>[2x]DPKFQRVALSDGHFIPVLGFGTYAPEEVPKSKAMEATKIAIDAGFRHIDSAYFYKNEKEVGLAIRSKIADGTVKREDIFYTSKLWCTFHRPELVRPSLEDSLKNLQLDYVDLYIIHFPTALKPGVEIIPTDEHGKAIFDTVDICATWEAMEKCKDAGLAKSIGVSNFNRRQLEMILNKPGLKYKPVCNQVECHPYLNQGKLLEFCKSKGIVLV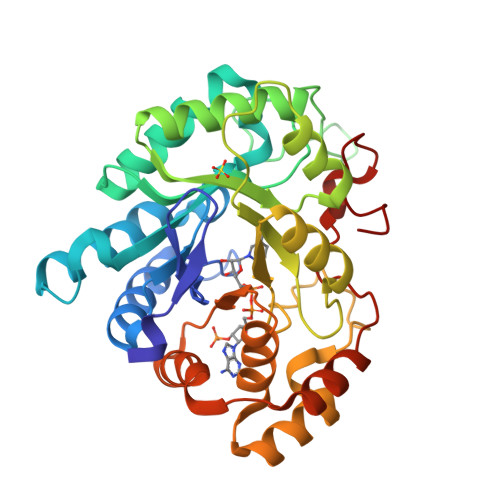AYSALGSHREPEWVDQSAPVLLEDPLIGALAKKHQQTPALIALRYQLQRGIVVLAKSFTEKRIKENIQVFEFQLPSEDMKVIDSLNRNFRYVTADFAIGHPNYPFSDEY> TIEKRYDFVFLFDVQDGNPNGDPDAGNLPRIDPQTGEGLVTDVCLKRKVRNFIQMTQNDEHHDIFIREKGILNNLIDEAHEQENVKGKEKGEKTEAARQYMCSRYYDIRTFGAVMTTGKNAGQVRGPVQLTFSRSIDPIMTLEHSITRMAVTNEKDASE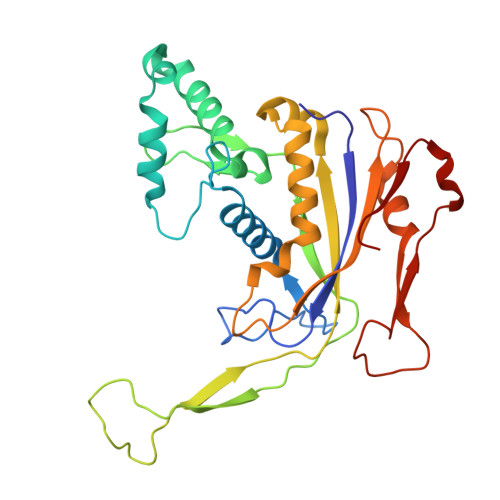TGDNRTMGRKFTVPYGLYRCHGFISTHFAKQTGFSENDLELFWQALVNMFDHDHSAARGQMNARGLYVFEHSNNLGDAPADSLFKRIQVVKKDGVEVVRSFDDYLVSVDDKNLEETKLLRKLGG{(2R)-7-nitro-2-[(propan-2-ylamino)methyl]-1,2,3,4-tetrahydroquinolin-6-yl}methanol 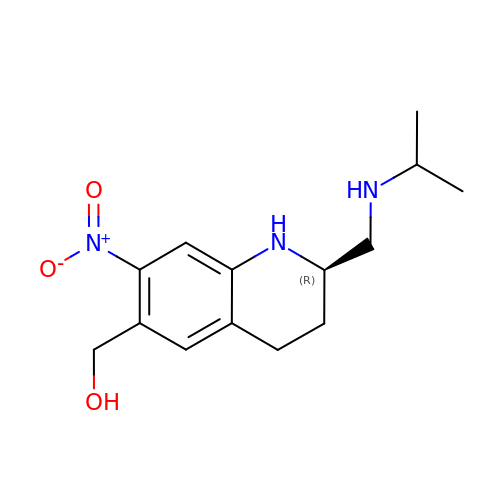| C14 H21 N3 O3 | XCGYUJZMCCFSRP-GFCCVEGCSA-N> MGHHHHHHHSSENLYFQGHMRKIRVGLIFGGKSAEHEVSLQSARNILDALDPQRFEPVLIGIDKQGQWHVNDPDSFLLHADDPARIALHRSGRGVALLPGAQQQQLRPIQPEQALAQIDVVFPIVHGTLGEDGSLQGLLRMANLPFVGSGVLGSAVAMDKDMAKRVLRDARLAVAPFVCFDRHTAAHADVDTLIAQLGLPLFVKPANQGSSVGVSQVRTADAFAAALALALAYDHKVLVEAAVAGREIECAVLGNAVPHASVCGEVVVHDAFYSYATKYISEHGAEIVIPADIDAQTQQRIQQIAVQAYQALG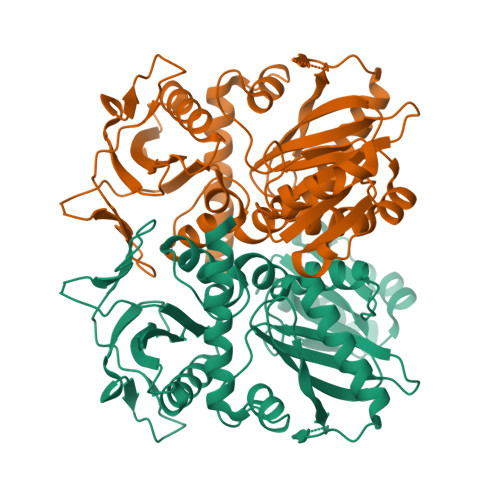CAGMARVDVFLCADGRIVINEVNTLPGFTRISVYPKLWQASGLDYRGLITRLIELALERHTDDQLLRSAVELH> TYFITMNNARNFFIQQLESNAQDTATSLGLSLSQSLINHDVPTMDSMVKAVFDRGYFSSIKVQDIKGKVIILKKQLPQESDIPQWFVNLIKWPSTEKSSLIMDGWMQAGVVLVASDPSYVYASLWRNAVEM

LapD is a c-di-GMP receptor that translates changes in the concentration of this cytosolic second messenger into cell-surface events via an inside-out signaling mechanism that ultimately controls cell adhesion. Specifically, c-di-GMP-bound LapD engages the periplasmic protease LapG through its Per-Arnt-Sim (PAS)-like domain, preventing it from cleaving the cell surface-bound large adhesin LapA, a protein mediating cell adhesion to multiple substrates. In contrast, c-di-GMP-unbound LapD adopts an autoinhibited conformation and loses its affinity for LapG. To address these shortcomings, we report here two structures, that of the output domain of a LapD ortholog from L. pneumophila, also known and referred to here as CdgS9, and that of LapG in complex with the same output domain.

The structure of L. pneumophila CdgS9Output (residues of 22–152) was determined from data collected on a crystal grown from selenomethionine-derivatized protein by using single anomalous dispersion (SAD) phasing (see ‘Material and methods’). The asymmetric unit contains one molecule of CdgS9Output, which adopts a PAS-like domain fold with the highest structural homology to CitA. A potential biologically relevant dimer involves a crystallographic symmetry mate, burying 3020 Å2 surface area at the twofold symmetry axis via favorable interactions (estimated ΔGint = −20.2 kcal/mol). The protomers form a parallel dimer, with the termini lining up at one end of the complex, consistent with their connectivity to the transmembrane helices that flank the periplasmic domain. CdgS9Output adopts a ‘parallel’ conformation as opposed to the open, V-shaped form that we observed in case of LapDOutput. As a consequence, the tryptophan residues (W125 in P. fluorescens LapD; W126 in L. pneumophila CdgS9) that form the distal tip of the PAS fold and appear to be a main anchor point for LapG binding are farther apart in the P. fluorescens dimer than the L. pneumophila LapD ortholog (50 Å vs 35 Å between their respective Cβ positions). Taken together, the cross-linking data clearly indicate that the topology observed in the CdgS9Output structure represents the biologically relevant model, which is conserved in the two LapD orthologs, LapD and CdgS9, despite only moderate overall sequence conservation (31% identity/52% similarity). In the apo-state, the output domain dimer of CdgS9 contains central four-helix bundles, either via packing of helices α1 and α2 of the PAS domain fold close to the distal end, or helices α1 and α4 at the membrane-proximal region. Closer to the membrane, a cluster of 4 phenylalanine residues (2 per protomer; F33 and F34 of CdgS9) stack in a perpendicular fashion, as opposed to the packing near the distal tip, which involves the burying of two symmetry-related arginine residues (R75 of CdgS9). High-affinity LapG binding to the off-state of LapD is prevented by an apparent surface mismatch.> MTVTRRHFLKLSAGAAVAGAFTGLGLSLAPTVARAELQKLQWAKQTTSICCYCAVGCGLIVHTAKDGQGRAVNVEGDPDHPINEGSLCPKGASIFQLGENDQRGTQPLYRAPFSDTWKPVTWDFALTEIAKRIKKTRDASFTEKNAAGDLVNRTEAIASFGSAAMDNEECWAYGNILRSLGLVYIEHQARIUHSPTVPALAESFGRGAMTNHWNDLANSDCILIMGSNAAENHPIAFKWVLRAKDKGATLIHVDPRFTRTSARCDVYAPIRSGADIPFLGGLIKYILDNKLYFTDYVREYTNASLIVGEKFSFKDGLFSGYDAANKKYDKSMWAFELDANGVPKRDPALKHPRCVINLLKKHYERYNLDKVAAITGTSKEQLQQVYKAYAATGKPDKAGTIMYAMGWTQHSVGVQNIRAMAMIQLLLGNIGVAGGGVNALRGESNVQGSTDQGLLAHIWPGYNPVPNSKAATLELYNAATPQSKDPMSVNWWQNRPKYVASYLKALYPDEEPAAAYDYLPRIDAGRKLTDYFWLNIFEKMDKGEFKGLFAWGMNPACGGANANKNRKAMGKLEWLVNVNLFENETSSFWKGPGMNPAEIGTEVFFLPCCVSIEKEGSVANSGRWMQWRYRGPKPYAETKPDGDIMLDMFKKVRELYAKEGGAYPAPIAKLNIADWEEHNEFSPTKVAKLMNGYFLKDTEVGGKQFKKGQQVPSFAFLTADGSTCSGNWLHAGSFTDAGNLMARRDKTQTPEQARIGLFPNWSFCWPVNRRILYNRASVDKTGKPWNPAKAVIEWKDGKWVGDVVDGGGDPGTKHPFIMQTHGFGALYGPGREEGPFPEHYEPLECPVSKNPFSKQLHNPVAFQIEGEKKAVCDPRYPFIGTTYRVTEHWQTGLMTRRCAWLVEAEPQIFCEISKELAKLRGIGNGDTVKVSSLRGALEAVAIVTERIRPFKIEGVDVHMVGLPWHYGWMVPKNGGDTANLLTPSAGDPNTGIPETKAFMVDVRKVWSHP;> MGKMFFVDLSRCTACRGCQIACKQWKNLPAEETRNTGSH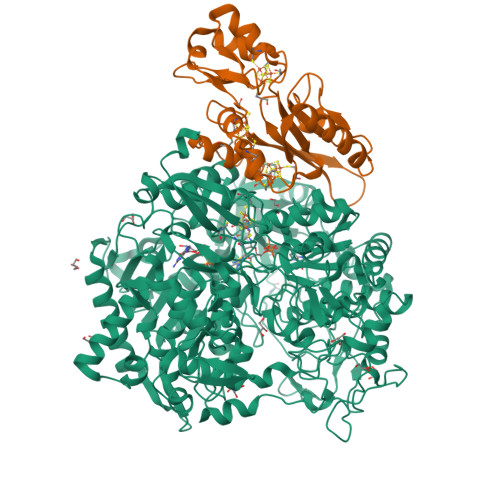QNPPDLSYVTLKTVRFTEKSRKGPGIDWLFFPEQCRHCVEPPCKGQADVDLEGAVVKDETTGAVLFTELTAKVDGESVRSACPYDIPRIDPVTKRLSKCDMCNDRVQNGLLPACVKTCPTGTMNFGDEQEMLALAEKRLAEVKKTYPGAVLGDPNDVRVVYLFTRDPKDFYEHAVADLAPSMMTRQQLFARLFRPRA>[2x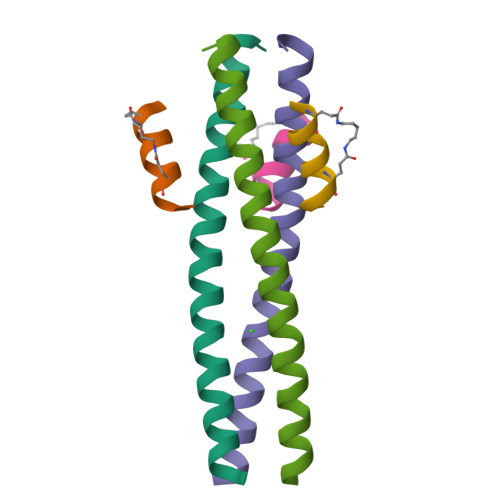]XRMKQIEDKIEEIESKQKKIENEIARIKKLLQLTVWGIKQLQARIL;>[2x]WEEWDREIENYT> NEHHHETMSEAQPQ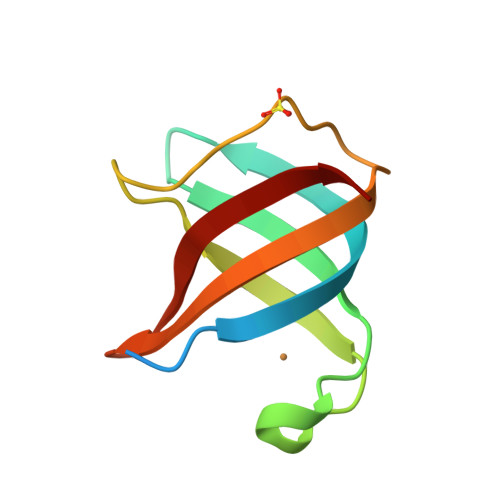VISATGVVKGIDLESKKITIHHDPIAAVNWPEMTMRFTITPQTKMSEIKTGDKVAFNFVQQGNLSLLQDIKVSQ> MQVTHSMPPQKLEIFKSLDDWARNNVLIHLKSVEKSWQPQDYLPDPVSDGFEEQVRELRERAKEIPDDYFVVLVGDMITEEALPTYMSMLNRCDGIKDETGAEPSAWAMWTRAWTAEENRHGDLLNKYLYLSGRVDMRKIEKTIQYLIGSGMDIKSENSPYLGFIYTSFQERATFISHANTAKLAQHYGDKKLAHICGSIASDEKRHATAYTKIVEKLAEIDPDTTVIAFADMMRKKITMPAHLMYDGSDELLFK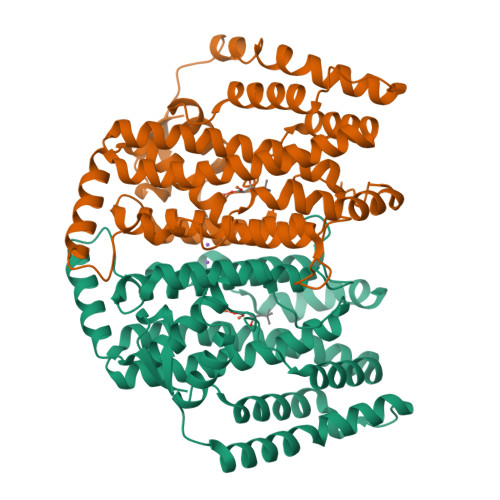HFTAVAQRLGVYSALDYCDILEFLVDKWNVERLTGLSDEGRKAQEYVCELGPKIRRLEERAQGRAKEAPTMPFSWIFDRQVKL;> MQVTHSMPPQKLEIFKSLDDWARNNVLIHLKSVEKSWQPQDYLPDPVSDGFEEQVRELRERAKEIPDDYFVVLVGDMITEEALPTYMSMLNRCDGIKDETGAEPSAWAMWTRAWTAEENRHGDLLNKYLYLSGRVDMRKIEKTIQYLIGSGMDIKSENSPYLGFIYTSFQERATFISHANTAKLAQHWGDKNLAHICGSIASDEKRHATAYTKIVEKLAEIDPDTTVIAFADMMRKKITMPAHLMYDGSDELLFKHFTAVAQRVGVYSALDYCDILEFLVDKWNVERLTGLSDEGRKAQEYVCELGPKIRRLEERAQGRAKEAPTMPFSWIFDRQVKL>[2x]GPDSENGVGDAELRERLRQCEETIEQLRAENQELKRKLNILTRPSGILVNDTKLDGPILQILFMNNAISKQYHQEIEEFVSNLVKRFEEQQKNDVEKTSFNLLPQPSSIVLEEDHKVEESCAIKNNKEAFSVVGSVLYFTNFCLDKLGQPLLNENPQLSEGWEIPKYHQVFSHIVSLEGQEIQVKAKRPKPHCFNCGSEEHQMKDCPMPRNAARISEKRKEYMDACGEANNQNFQQRYHAEEVEERFGRFKPGVISEELQDALGVTDKSLPPFIYRMRQLGYPPGWLKEAELENSGLALYD;>[2x]GPDSMADAFGDELFSVFEGDSTTAAGTKKDKEKDKGKWKGPPGSADKAGKRFDGKLQSESTNNGKNKRDVDFEGTDEPIFGKKPRIEESITEDLSLADLMPRVKVQSVETVEGCTHEVALPAEEDYLPLKPRVGKAAKEYPFILDAFQREAIQCVDNNQSVLVSAHTSAGKTVCAEYAIALALREKQRVIFTSPIKALSNQKYREMYEEFQDVGLMTGDVTINPTASCLVMTTEILRSMLYRGSEVMREVAWVIFDEIHYMRDSERGVVWEETIILLPDNVHYVFLSATIPNARQFAEWICHLHKQPCHVIYTDYRPTPLQHYIFPAGGDGLHLVVDENGDFREDNFNTAMQVLRDAGDLAKGDQKGRKGGTKGPSNVFKIVKMIMERNFQPVIIFSFSKKDCEAYALQMTKLDFNTDEEKKMVEEVFSNAIDCLSDEDKKLPQVEHVLPLLKRGIGIHHGGLLPILKETIEILFSEGLIKALFATETFAMGINMPARTVLFTNARKFDGKDFRWISSGEYIQMSGRAGRRGMDDRGIVILMVDEKMSPTIGKQLLKGSADPLNSAFHLTYNMVLNLLRVEEINPEYMLEKSFYQFQHYRAIPGVVEKVKNSEEQYNKIVIPNEESVVIYYKIRQQLAKLGKEIEEYIHKPKYCLPFLQPGRLVKVKNEGDDFGWGVVVNFSKKSNVKPNSGELDPLYVVEVLLRCSKESLKNSATEAAKPAKPDEKGEMQVVPVLVHLLSAISSVRLYIPKDLRPVDNRQSVLKSIQEVQKRFPDGIPLLDPIDDMGIQDQGLKKVIQKVEAFEHRMYSHPLHNDPNLETVYTLCEKKAQIAIDIKSAKRELKKARTVLQMDELKCRKRVLRRLGFATSSDVIEMKGRVACEISSADELLLTEMMFNGLFNDLSAEQATALLSCFVFQENSSEMPKLTEQLAGPLRQMQECAKRIAKVSAEAKLEIDEETYLSSFKPHLMDVVYTWATGATFAHICKMTDVFEGSIIRCMRRLEELLRQMCQAAKAIGNTELENKFAEGITKIKRDIVFAASLYL

The nuclear exosome targeting (NEXT) complex plays a central role in directing non-functional transcripts to exosome-mediated degradation, but the structural and molecular mechanisms remain enigmatic. Here, we elucidated the architecture of the human NEXT complex, showing that it exists as a dimer of MTR4-ZCCHC8-RBM7 heterotrimers. Dimerization preconfigures the major MTR4-binding region of ZCCHC8 and arranges the two MTR4 helicases opposite to each other, with each protomer able to function on many types of RNAs. In terms of architecture, we found that the biological unit of NEXT consists of two copies of each MTR4 and RBM7, assembling symmetrically around a highly intertwined ZCCHC8 homodimer, with an arrangement conducive for targeting different RNA substrates.

The smaller version of NEXT (defined as NEXTS) consisted of full-length MTR4, a truncated mutant of RBM7 containing the RRM domain (residues 1–98, for simplicity referred to as RBM7; Falk et al., 2016), and a truncated mutant of ZCCHC8 in which only the minimal MTR4- and RBM7-binding regions remained (residues 41–337, referred to as ZCCHC8S; Falk et al., 2016). The cryo-EM analysis of the NEXTS complex resulted in a reconstruction with a global resolution of 4.5 Å. The map showed ordered density for two MTR4 protomers (referred to as MTR4A and MTR4B) facing each other in a head-to-head configuration. This density was separately fitted with the atomic models of the MTR4 DExH-box domain and arch domain, as the latter has different conformations in the available crystal structures (Lingaraju et al., 2019a; Wang et al., 2019; Puno and Lima, 2018). In our reconstruction of NEXTS, the MTR4 arch domain of both protomers is arranged in an inward conformation, similar to that observed in apo human MTR4 (Wang et al., 2019) and apo yeast Mtr4 (Weir et al., 2010). The KOW domains of the two MTR4 helicases sandwich a globular density that is, in turn, connected to an elongated protrusion. Briefly, NEXT forms a homodimer built around the N-terminal region of two ZCCHC8 protomers, which intertwine to form a coiled coil and a globular dimerization module. The ZCCHC8 dimerization module interacts in a symmetric manner with two MTR4 protomers via their arch domains, in turn positioning the DExH-box helicase domains in opposing orientations with respect to each other. The cryo-EM analysis of NEXTS allowed visualization of the interaction between the ZCCHC8 N-terminal dimerization module and the MTR4 KOW domain but failed to reveal other features of the complex (e.g., the RBM7 binding site), most likely due to their inherent flexibility.>[2x]CGCGCG

In this paper, we describe an ultrahigh-resolution crystal structure of Z-DNA with the sequence l-d(CGCGCG)2, in which the natural 2′-deoxy-d-ribose was replaced with its l-enantiomer. Natural d-deoxyoligonucleotides [for example d-d(CGC­GCG)2; d-DNA] and their synthetic enantiomers [l-d(CGC­GCG)2, l-DNA] with the same sequence have the same physical (for example duplex stability or solubility) and chemical properties. The l-enantiomers are also resistant to nuclease degradation and to many off-target interactions that plague traditional d-oligonucleotide-based technologies. Cadaverine2+ [Cad2+; ], a biogenic amine, is a positively charged organic dication under physiological ionic and pH conditions and hence can interact with negatively charged macromolecules such as DNA and RNA.

The self-complementary l-d(CGCGCG)2 purine/pyrimidine hexanucleotide was crystallized in complex with the polyamine cadaverine and potassium cations. Since the oligonucleotide contained the enantiomeric 2′-deoxy-l-ribose, the Z-DNA duplex is right-handed, as confirmed by the ultrahigh-resolution crystal structure determined at 0.69 Å resolution. The sugar-phosphate backbone assumes two conformations, but the base pairs do not show any sign of disorder. Within the DNA molecule, two alternative conformations (labeled I and II) are clearly visible in the electron-density map at the inter-nucleotide phosphate linkages between C3–G4, G4–C5, C5–G6 and G8–C9, the refined occupancies of which converged at 0.575 (21)/0.425 (22), 0.556 (6)/0.444 (6), 0.597 (13)/0.403 (13) and 0.80 (12)/0.20 (12), respectively. Here, the ZII conformation of the phosphate group can only be assigned to G4(I), with ζ = 62.7° (the signed ζ torsion angle is given for the reference 2′-deoxy-d-ribose enantiomer). This alternative ZII conformer is stabilized by hydrogen bonds to the N1 atom of Cad2+ and a water molecule. As illustrated by our structure, this assumption is especially true for Cad2+, where the N1+⋯N2+ distance of 7.451 (23) Å allows the formation of four hydrogen bonds to adjacent phosphate groups of the Z-DNA duplex (in the ideal Z-DNA hexamer, the P⋯P distances are in the range ∼5.69 to ∼7.18 Å). The K+ cation, with an occupancy of 0.32, has an irregular coordination sphere that is formed by three OP atoms of two symmetry-related Z-DNA duplexes and one O5′ hydroxyl O atom, and is completed by three water sites, one of which is twofold disordered.> SGLVPRGSHMMEILRGSP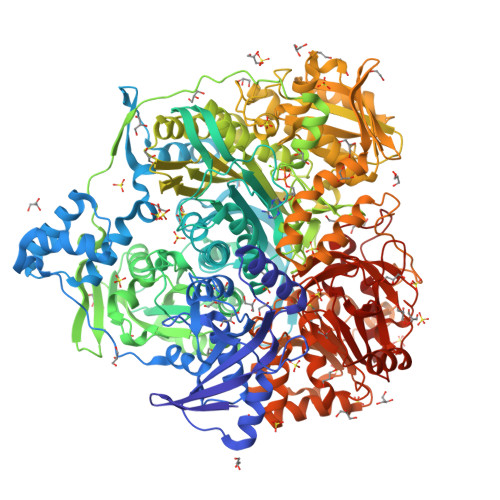ALSAFRINKLLARFQAANLQVHNIYAEYVHFADLNAPLNDSEQAQLTRLLQYGPALSSHTPAGKLLLVTPRPGTISPWSSKATDIAHNCGLQQVDRLERGVAYYIEASTLTAEQWRQVAAELHDRMMETVFSSLTDAEKLFIHHQPAPVSSVDLLGEGRQALIDANLRLGLALAEDEIDYLQEAFTKLGRNPNDIELYMFAQANSEHCRHKIFNADWIIDGKPQPKSLFKMIKNTFETTPDYVLSAYKDNAAVMEGSAVGRYFADHNTGRYDFHQEPAHILMKVETANHPTAISPWPGAATGSGGEIRDEGATGRGAKPKAGLVGFSVSNLRIPGFEQPWEEDFGKPERIVTALDIMTEGPLGGAAFNNEFGRPALTGYFRTYEEKVNSHNGEELRGYHKPIMLAGGIGNIRADHVQKGEIVVGAKLIVLGGPAMNIGLGGGAASSMASGQSDADLDFASVQRDNPEMERRCQEVIDRCWQLGDANPILFIHDVGAGGLSNAMPELVSDGGRGGKFELRDILSDEPGMSPLEIWCNESQERYVLAVAADQLPLFDELCKRERAPYAVIGDATEEQHLSLHDNHFDNQPIDLPLDVLLGKTPKMTRDVQTLKAKGDALNRADITIADAVKRVLHLPTVAEKTFLVTIGDRTVTGMVARDQMVGPWQVPVADCAVTTASLDSYYGEAMSIGERAPVALLDFAASARLAVGEALTNIAATQIGDIKRIKLSANWMAAAGHPGEDAGLYDAVKAVGEELCPQLGLTIPVGKDSMSMKTRWQEGNEQREMTSPLSLVISAFARVEDVRHTLTPQLSTEDNALLLIDLGKGHNALGATALAQVYRQLGDKPADVRDVAQLKGFYDAMQALVAARKLLAWHDRSDGGLLVTLAEMAFAGHCGVQVDIAALGDDHLAALFNEELGGVIQVRAEDRDAVEALLAQYGLADCVHYLGQALAGDRFVITANDQTVFSESRTTLRVWWAETTWQMQRLRDNPQCADQEHEAKANDTDPGLNVKLSFDINEDIAAPYIATGARPKVAVLREQGVNSHVEMAAAFHRAGFDAIDVHMSDLLGGRIGLGNFHALVACGGFSYGDVLGAGEGWAKSILFNHRVRDEFETFFHRPQTLALGVCNGCQMMSNLRELIPGSELWPRFVRNHSDRFEARFSLVEVTQSPSLLLQGMVGSQMPIAVSHGEGRVEVRDDAHLAALESKGLVALRYVDNFGKVTETYPANPNGSPNGITAVTTENGRVTIMMPHPERVFRTVANSWHPENWGEDSPWMRIFRNARKQLG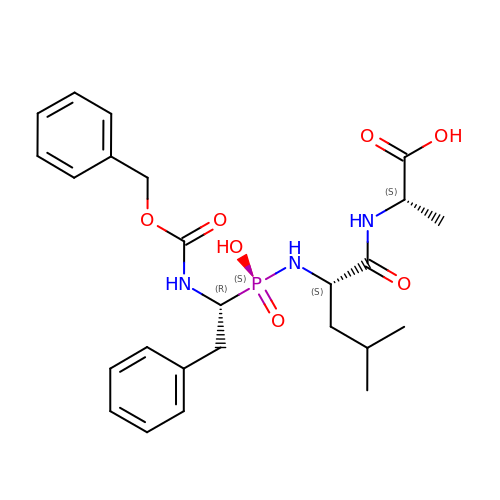N-[(S)-[(1R)-1-{[(benzyloxy)carbonyl]amino}-2-phenylethyl](hydroxy)phosphoryl]-L-leucyl-L-alanine | C25 H34 N3 O7 P | PREBTZMCCRSQJI-YUXAGFNASA-N>SKPFTIPILTIGEMTNSRFPVAIDMLHTSPTDNFIVQPQNGRCTLDGELQGTTQLVASNICAFRGSISGHENNGDQHQWHFSITNPNGTPFDPTEDVPAPLGTPDFKGQLYGVISQRNREGSSGNGNQKANRSHEGVISTVAPRFTPKLGSVMIGTWTTDDIQDQPSRFTPVGLNDDDNYKQWELPNYSGALTLNMGLAPSVFPTYPGEQLLFFRSYIPMKGGYGSPYIDCLIPQEWISHFYQESAPSQTDVALIRYVNPDTGRVLFEAKLHRQGYITVAKTGDSPINVPANGYFRFDSWVSQFYSLAPM[2x]

Noroviruses are highly contagious, infecting both humans and animals. The human norovirus capsid protruding (P) domain binds histo-blood group antigen (HBGA) co-factors for infection, and a recently discovered bat norovirus (GX) was also found to interact with HBGAs. In this study, we determined the P domain structures of four human noroviruses and one bat norovirus using X-ray crystallography to examine structural features linked to potential interspecies transmission. The principal structural difference was a variable length P2 subdomain loop (Loop A), which was located near the HBGA pocket.

The P domains of GII.9 (AY038599), GII.23 (KT290889), GII.27 (MG495077), GVIII (AJ844470), and GX (MF373609) were expressed in E.coli. The five P domains were structurally equivalent with a root mean square deviation for C-alpha atoms ranging between 0.586 Å (GII.23-GII.27) and 1.645 Å (GII.9-GX). The cross-reactivity of the P domains was determined using direct ELISA with a broad-spectrum human norovirus Nanobody (Fc-NB26) that binds to a highly conserved region on the P domain. Fc-NB26 bound to GII.9, GII.23, and GII. P domains in a dose-dependent manner at concentrations less than 80 ng/mL. Structural modeling of the Fc-NB26-binding site indicated that GII.9, GII.23, and GII. P domains contained most of the equivalent residues that could interact with Fc-NB26. Our cumulative data show that Fc-NB26/NB26 binds most GII genotypes, and the epitope is vulnerable and a therapeutic target region for GII noroviruses.> MASMTGGQQMGRGSMSRDP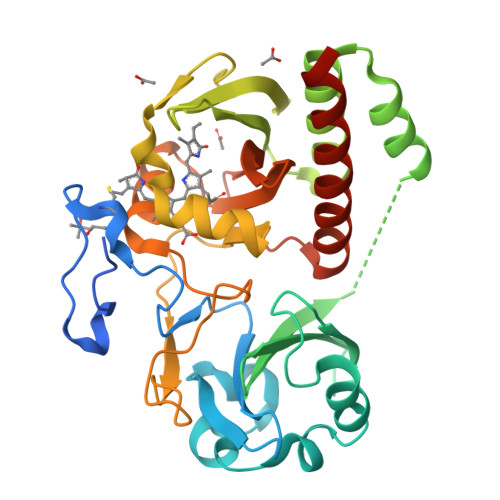LPFFPPLYLGGPEITTENCEREPIHIPGSIQPHGALLTADGHSGEVLQMSLNAATFLGQEPTVLRGQTLAALLPEQWPALQAALPPGCPDALQYRATLDWPAAGHLSLTVHRVGELLILEFEPTEAWDSTGPHALRNAMFALESAPNLRALAEVATQTVRELTGFDRVMLYKFAPDATGEVIAEARREGLHAFLGHRFPASDIPAQARALYTRHLLRLTADTRAAAVPLDPVLNPQTNAPTPLGGAVLRATSPMHMQFLRNMGVGSSLSVSVVVGGQLWGLIACHHQTPYVLPPDLRTTLEYLGRLLSLQVQVKEALEHHHHHH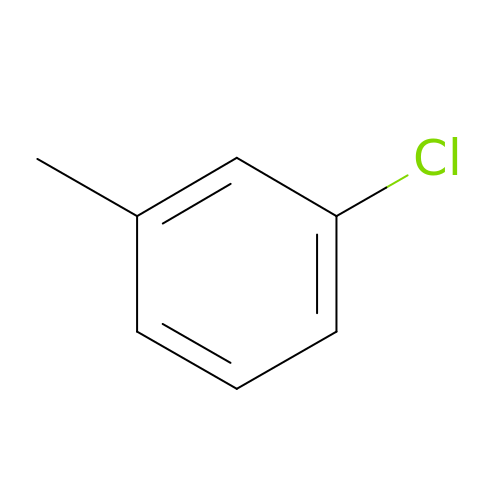1-chloranyl-3-methyl-benzene | C7 H7 Cl | OSOUNOBYRMOXQQ-UHFFFAOYSA-N> SMDLRVQELIKLICNVQAMEEMMMEMKYNTKKAPLGKLTVAQIKAGYQSLKKIEDCIRAGQHGRALMEACNEFYTRIPHDFGLRTPPLIRTQKELSEKIQLLEALGDIEIAIKLVKTELQSPEHPLDQHYRNLHCALRPLDHESYEFKVISQYLQSTHAPTHSDYTMTLLDLFEVEKDGEKEAFREDLHNRMLLWHGSRMSNWVGILSHGLRIAHPEAPITGYMFGKGIYFADMSSKSANYCFASRLKNTGLLLLSEVALGQCNELLEANPKAEGLLQGKHSTKGLGKMAPSSAHFVTLNGSTVPLGPASDTGILNPDGYTLNYNEYIVYNPNQVRMRYLLKVQFNFLQLW

The human diphtheria toxin-like ARTD family contains PARP and tankyrase (TNKS) enzymes that can catalyze both mono-ADP-ribosylation (MAR, mono-ARTs) as well as generate elongated and branched chains of poly-ADP-ribose (PAR, poly-ARTs). The PARPs and TNKSs form a family of structurally and functionally diverse enzymes, which are involved in the regulation of various key biological and pathological processes such as DNA repair, cell differentiation, gene transcription, and signal transduction pathways. PARPs and TNKSs use nicotinamide adenine dinucleotide, NAD+, to transfer an ADP-ribose (ADPr) unit onto target proteins or nucleic acids with the release of nicotinamide. Here, we report our contribution in identifying a set of compounds based on a new nicotinamide mimicking chemotype, [1,2,4]triazolo[3,4-b]benzothiazole (TBT), able to inhibit different PARP family enzymes with submicromolar activity depending on the substitution pattern around the central core. The binding mode of the TBT scaffold was studied through the synthesis of analogues and their complex crystal structures with PARP2, TNKS2, PARP14, and PARP15.

On the contrary, hydroxy derivative 16 (OUL245) inhibits poly-ARTs with a selectivity toward PARP2. Interestingly, the presence of a C-7 hydroxy group made 16 very potent and specific for poly-ARTs with nearly 10-fold selectivity for PARP2 over TNKS2 (IC50 of 44 vs 370 nM). Based on the comparison of complex structures of PARP2 and PARP15, 16 has a similar binding mode as 1, but the catalytic residue of PARP2 (Glu558), not present in PARP15, interacts with the hydroxyl group of 16. The hydroxyl group also interacts with the Met456 backbone amide via a water molecule. In addition, 16 showed μM IC50 values for the other active site glutamate containing mono-ARTs PARP3–4. This is consistent with the crystal structures where the hydroxyl of 16 forms a hydrogen bond with the glutamate. 7-Hydroxy derivative 16 is of special interest as a poly-ART inhibitor since it is both a potent (IC50 = 44 nM) and specific PARP2 inhibitor with 13-fold selectivity over PARP1. Structurally, PARP1 and PARP2 are both able to form the same interactions with the hydroxy moiety, and therefore, there is no apparent reason for the observed selectivity.>ASVSARTLHFGTSATYAPYEFVDADNKIVGFDIDVANAVCKEMQAECSFTNQSFDSLIPSLRFKKFDAVIAGMDMTPKREQQVSFSQPYYEGLSAVVVTRKGAYHTFADLKGKKVGLENGTTHQRYLQDKQQAITPVAYDSYLNAFTDLKNNRLEGVFGDVAAIGKWLKNNPDYAIMDERA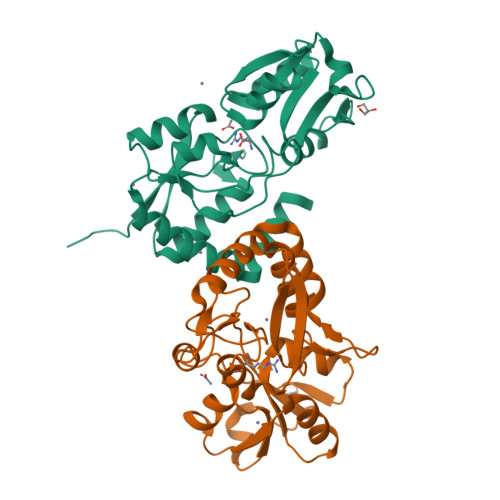SDPDYYGKGLGIAVRKDNDALLQEINAALDKVKASPEYAQMQEKWFTQ[2x]>C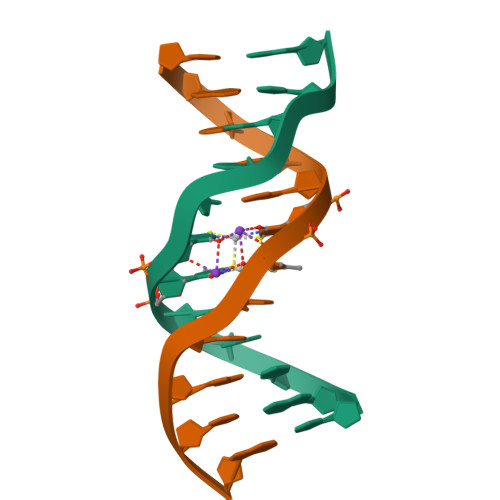GCGAXXTCGCG[2x]Here, we report the cryo-EM structure of the cyanophage P-SCSP1u, a representative member of the MPP-C phages, in its native form at near-atomic resolution, which reveals the assembly mechanism of the capsid and molecular interaction of the portal-tail complex. Overall, the P-SCSP1u virion possesses an icosahedral capsid with a diameter of ~600 Å and a short tail of ~190 Å in length. The recently identified MPP-C (Marine Picocyanobacteria Podovirus clade C) cyanophages, belonging to the T7-like podoviruses, contain the smallest genomes among cyanopodoviruses and exhibit distinct infection kinetics. By using single-particle cryo-EM, we finally determined the structure of P-SCSP1u in its native state at 3.2 Å and 3.8 Å for the capsid and portal-tail complex, respectively.

The portal-tail complex of P-SCSP1u consists of dodecameric portal protein (gp16), dodecameric adaptor protein (gp22), hexametric nozzle protein (gp23), and hexametric trimer of fiber proteins (gp28), in a similar organization to those of T729,32 and the MPP-B cyanophage P-SSP723. By using the symmetry-mismatch reconstruction method, the asymmetrical portal-tail complex of P-SCSP1u was reconstructed to 3.8 Å resolution, enabling us to study the detailed assembly between each subunit. The cylinder-shaped P-SCSP1u portal, 170 Å in height with the largest external diameter of 160 Å, is formed by 12 copies of gp16 that are arranged around an axial central channel. Similar to the portal protein of T7 (gp8), the portal protein of P-SCSP1u is composed mainly of α-helices and can be divided into five domains: C-terminal helical barrel, crown, wing, stem, and clip. The clip regions of the portal provide a basis for connecting 12 copies of the adaptor protein gp22, which bridge all other components in the portal-tail complex. Each of the six fiber trimers of P-SCSP1u (gp28) is fitted between the nozzle fiber dock and the adaptor fiber dock. The platform region of N1 tightly interacts with the helix bundle regions of A2 and A3 by two pairs of hydrogen bonds (R766-E20 and D737-N24) and one pair of salt bridges (R766-E19). Collectively, the dodecameric portal, dodecameric adaptor, and the hexametric nozzle in the portal-tail complex are intimately connected with each other, with a total of 60 hydrogen bonds and 18 salt bridges, providing a stable platform for DNA ejection. The succeeding loop of the dodecameric portal protein constitutes one of the narrowest sections of the channel, which was previously identified as a “valve” and suggested to function as clamps to retain packaged DNA in the phage T732. According to the radii of the channels, an additional narrow “valve”, which we named valve S, is identified in the P-SCSP1u capsid. Intriguingly, an additional gate, which we named gate 1S, is identified in the middle of the nozzle located between gates 1 and 2.

>[6x]MPLISSSIPNLINGVSQQPAALRLASQAEEVINCMPSPVEGLKKRPPMQHIKKLFAGSAGTGRPFTHIVDRDGVIRYLIFIQDNAIKVFDLDGNAQTVSTPNGTSYLNITGEPSSTFRVASIADFTFIVNREKTVAMDTTNKSYNWGTKSMVFIKSADFSTTYRVKLNGTEKSVTTGNSSGSAPDTVTIASDLATQLNTISGFTVTSTDYIIRITKDDGGDYTLESSDTKTADATSAIKGTVDSITDLPTIAEHNFTVRIQGSATTAFDDYFVKFEATAGSGFGPGVWRETVAPNIDHLLDKSTMPHTLVRNANGTFTFAQFNYTGRVAGDTTTAPNPTFVGSKIKNINLFRNRLVFLADENVILSAADSFERFFPETVQTLLDSDPIDISSGGTSVNFLNSSLAFANTLLLFSLHGQFRLDTGSTSVGTALTPKTATITAITTFDIVDAIDPIGVGRTVYFGIPKGDFSGLREYFLPDASGPIPLSEEVTSSVPRFVPGNLISMSPSVSEEVITMISKDQPRRVYIYKFFFDDDQKLQSSWSYWEVAANKTLLGGNVLDSDLYTCVEYSDGVYLEKTQLRPETVDSGTEFEILLDRKTTEAACSTSLINSGALGVQTVITLPYPMSGTGTMAVVGRFASNNTIAHGQVIKATAETLTGGASGNGTMTVPGDLSSAKFFVGEIYNMTYEFSTPYLKETPPGGGLAVLANPRLQLRTWSIVFDETSNFSMKITPGQRDELTYPFNGYKIGSGQFPIGTPSLATGRFRVPVMAQNIETKIVLFSDSPLPCRVQSAEWEGWYQERARRL;>MAARTSFLDAVNRVLQMLGEAPVNSLQGQFGLAKQAEVALNDVSRTIQTEGWSFNTDLEKKLERNSSNEIELSSNVSRVVVDNLEYPDIDVVQRGDKLYDRKNNRYTFDEDLIVDMTTILEWDLLPEHARQYITIKAGRQLQEAIIGSAELTKLNLTQEVEARSAFLEEETTKSEHSMLRGHLNRTSPVNTYIPSRTLER[12x];>MAFAQRIITSNSAGDQEFTFTFDYIKEEHIKVFVNFVEKAQGTGSNEFQVITNTTPKKISLNTGLSADNTRVEIRRVSSLSTPLVDFADGSTLTAADLDTAEKQSLFIDQELDDALKQGISIDTSTGVPTLNSQRLSNVSDPVNAQDAVTKAYLERSGSITSTQILNGTIVDADINASAAIAKSKLAALNIVNADVNASAAIAGSKLADASIAYTKIQNVSATNRILGRDSSGAGVIEEITPANLRTMINVEDGATADQSAAEIRTLVESASDSNVFTDADHTKLNAIEASADVTDATNVDAAGAVMNSDTSTAAMQFVIDEDTFGSNLDTKVPTQQSVKAYITATSQPLDSELSQLAGMQSGTASKLADSTALTADIADLNQLDGMAKETSITNSNTKFPTSAAVVNFVANQIAPVGGLEVIADEDSFPATQPVSGVVISISNADGLVINNAGEASNARTVGSGSDNVTIKNFPASLRNQTLAPNLGLLVSSTGASQEYNYHKLLAKETDVLQLSDDINDFNNRYRVENTLPAANDSSNHDGDLVYAKEEKKIYVYSGDYNGTPVGSFGEVQSIGNFFISTLSPAFNGSLQDFTITNAPSNAQQIILSINGVIQKPNSGTSTPSEGFALSGSTIKLAAAPPSGADYFAIVLGSTVNIGTPSNNTVTSSILQNGSVIEAKLGSGAVTRTKLNLVSTSSAPGLEVKGDGSSDGYLQLNCSQNSHGIKLKSPPHSAGQSYTLTFPSNIVSGQFLTTDANGNLSWAAVVTDLVNDTSPQLGGNLDCNDKNILLNDSSGSANNRIRLGASQDFALFHNGTINIIEAVSGDLHLRLNGSEEGIIVKQNGAVELYYDNSKKFHTSSVGATVTGNLFLSGGYINLNDNYSYGMGSGNRAQLYHSGNHQYLLNTVGNMYFQPKSGENGIVIIPDDAVELYHNNVKRLETTSGGVTVSGSVTATGHLFVGANTHYLYFTSTAGYSPRIGNADGGTGVNMTFHTNNTMRMMLQNDGHLRPASNNTYDLGTSSDRWRNVYTNDLNLSNEGGANDVDGTWGSYTIQEGAEDLFLINKRTSKKYKFNLTEVS[18x];>MKTRLTNNVDRQSALYGSSGGTAAQRYEQLRVDRNSPLKRARDCSKVTIPGLIEDENYGDAGRLDTPYQSSGARGVGHMTSKLAVTLFPTNEHFFKLEIDSLAILASDQNPEMITEFDSALVKVEQAVMRMFETIGGRAAMHEALKHLLVGGNVLLYVSDEGIKVIHLDSYVLCRDPMGNVTEIVVEEEIFKDALPEEYLDEEDDDDDDMGKKMVKIYTCIKFMDDQCHWYQEIKGKEVPGTHGKCAADVAPWIALRQDRVDSEMYGRSYVEQYYGDLLALENLYKAILEASASLSKVLFLCNPNGTTRPRTLSQASNGSIVQGNAADVTVLQAAGKSQDLQIANQTIERIENRLAFAFMLNTAIQRPGERVTAEEIRYMAQELDAGISGLYSILSRELQLPLVRRLIHILRRKRKLPDFPRSEVTGEPLIKEKAVTGIEAIGRGDDRNKLIDFITTANQALGPQAMTQFLNVEEALRRLAASGSIDTTNLVKTKAQLQQEAAAQAEAEQQAQQQQLLETGIKSPAMAQAVKNFQGADPERAAQALSAITSETGGIDADQLTEAV[12x]> AAQVLRGTVTDFPGFDERADAETLRKAAKGLGTDEESILTLLTSRSNAQRQEISAAFKTLFGRDLLDDLKSELTGKFEKLIVALAKPSRLYDAYELKHALKGAGTNEKVLTEIIASRTPEELRAIKQVYEEEYGSSLEDDVVGDTSGYYQRALVVLLQANRDPDAGIDEAQVEQDAQALFQAGELKWGTDEEKFITIFGTRSVSHLRKVFDKYATISGFQIEETIDRETSGNLEQLLLAVVKSIRSIPAYLAETLYYAAKGAGTDDHTLIRVAVSRSEIDLFNIRKEFRKNFA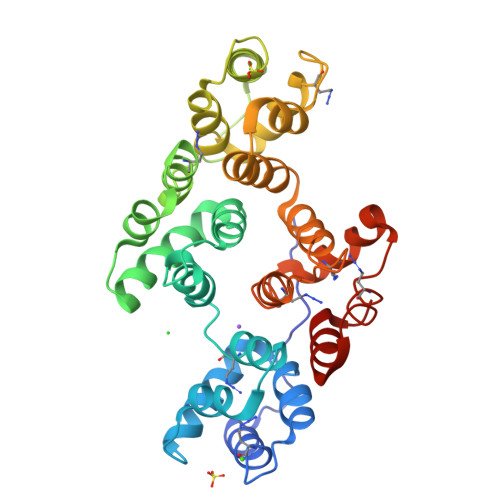TSLYSAIKGDTSGDYKKALLLLCGEDD>[2x]PREVLTGGHSVSAPQENRIYVMDSVFMHLTESRVHVYDYTNGKFLGMVPTAFNGHVQVSNDGKKIYTMTTYHERITRGKRSDVVEVWDADKLTFEKEISLPPKRVQGLNYDGLFRQTTDGKFIVLQNASPA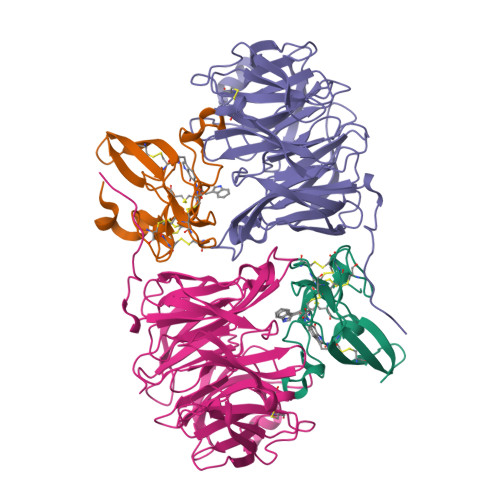TSIGIVDVAKGDYVEDVTAAAGCWSVIPQPNRPRSFMTICGDGGLLTINLGEDGKVASQSRSKQMFSVKDDPIFIAPALDKDKAHFVSYYGNVYSADFSGDEVKVDGPWSLLNDEDKAKNWVPGGYNLVGLHRASGRMYVFMHPDGKEGTHKFPAAEIWVMDTKTKQRVARIPGRDALSMTIDQQRNLMLTLDGGNVNVYDISQPEPKLLRTIEGAAEASLQVQFHPVGGT;>[2x]AGGGGSSSGADHISLNPDLANEDEVNSCDYWRHCAVDGFLCSCCGGTTTTCPPGSTPSPISWIGTCHNPHDGKDYLISYHDCCGKTACGRCQCNTQTRERPGYEFFLHNDVNWCMANENSTFHCTTSVLVGLA In Brassica, self/nonself-discrimination in the SI reaction is sporophytically controlled by a single locus, called S, with over 100 haplotypes (S1, S2, …, Sn). S receptor kinase (SRK), a receptor kinase containing an SLG-like ectodomain, transmembrane region, and intracellular kinase domain, acts as the pistil determinant. S-locus Protein 11 (SP11; also called SCR), a secreted small basic protein with four disulfide bonds forming a defensin-like structure, functions as the pollen determinant.

Here, we report the crystal structure of engineered S8-eSRK and S8-SP11 complex derived from S8-haplotype in B. rapa, which has a common overall structure with the S9-eSRK–S9-SP11 complex but an entirely different mode of the ligand recognition. Comprehensive protein engineering experiments yielded S8-eSRK containing 11 mutations (S8-meSRK) in two lectin domains that improved the expression of recombinant protein in the insect cell system. The crystal structure of the S8-meSRK ectodomain and chemically synthesized S8-SP11 complex was determined at 2.6 Å resolution. The complex, composed of a 2:2 S8-meSRK–S8-SP11 heterotetramer, forms a turned A-like structure. S8-meSRK consists of two lectin domains, an EGF-like domain, and a PAN domain with six disulfide bonds and three sugar chains. In the two SP11-binding sites of S8-meSRK, site 1 is 793.0 Å2 of the concaved surface area formed by all HV regions, and site 2 is a 444.1 Å2 crescent moon–like surface mainly formed by the HV II region. The β2–β3 loop of S8-SP11 forms a hydrogen bond network with the SP11-binding site 1 of S8-meSRK. The amino group of Lys63 in S8-SP11, located on the highly acidic concave surface of S8-meSRK, stabilizes the interaction. In SP11-binding site 2, the aromatic ring of Tyr275 in S8-meSRK is stacked with the plane of Asn65 side chain in S8-SP11, which forms three hydrogen bonds with Asn271, Glu277, and Ser293 of S8-meSRK. In the center of the dimerization surface in the S8-meSRK complex, His297, Val313, and Asn314 are in tight contact with the same residues of another S8-meSRK molecule via van der Waals interactions or hydrogen bonds.

>[2x]MQGVRYIYHHFYTSLLVFVVMILFRSALSIYINTLSSTESLTISNNRTLVSPGDVFELGFFTPGSSSRWYLGIWYKKLSERTYVWVANRDNPLSNSTGTLKISGNNLVLRGDSNKSIWSTNLTRGNERSPVVAELLANGNFVMRDSNNNDASGFLWQSFDYPTDTLLPEMKLGYDLKTGRNRFLTSSRNSDDPSSGDYSYKLEPRRLPEFYLLQGDVREHRSGPWNGIQFSGIPEDQKSSYMVYNFTENSEEVAYTFRMTNNSFYSRLTINSEGYLERLTWAPSSGAWNVFWSSPNHQCDMYRMCGPYSYCDVNTSPSCNCIQGFNPGNVQQWALRNQISGCKRRTRLSCNGDGFTRMKNIKLPDTRMAIVDRSIGLKECEKRCLSDCNCTAFANADIRNRVTGCVIWTGELEDMRNYAEGGQDLYVRLAAADSRLEVLFQGP;>RCTRGFRKLGKCTTLEEEKCKTLYPRGQCTCSDSKMNTHSCDCKSC[2x]ACs contain metal ions but not organic cofactors, and use ATP to activate substrates through phosphorylation. The first structural rationale for acetone carboxylation is presented here, focusing on the 360 kDa (αβγ)2 heterohexameric AC from Xanthobacter autotrophicus in the ligand-free, AMP-bound, and acetate coordinated states. Like many carboxylases, AC is a heteromultimeric enzyme complex. Its architecture consists of two heterotrimeric αβγ subunits joined by the interacting α-subunits to form a dimeric core.

In the absence of bound substrates or nucleotides (ligand-free form), the AC structure has an open cleft at the α/β subunit interface leading to the nucleotide-binding site in the β-subunit. The ligand-free structure is assigned as the resting state awaiting the binding of substrates ATP, acetone, and bicarbonate at the nucleotide-binding site. The ligand-free form of AC contains α-Glu89 positioned at the C-terminus of a Mn-proximal α-helix (residues α82–87) which blocks access to the Mn active site from the α/β interface. However, the structure of the native AC shows the nucleotide binding site located ~40 Å from the Mn site of acetoacetate formation, with no visible pathway for the transfer of reactive phosphorylated intermediates.

>[2x]MNVTVDQSTLAGATRGIVRGGETLKEHRDRLMAATKATGRYAGLKTLELREREPILYNKLFSRLRAGVVDARETAKKIAASPIVEQEGELCFTLYNAAGDSLLTSTGIIIHVGTMGAAIKYMIENNWEANPGVHDKDIFCNNDSLIGNVHPCDIHTIVPIFWEGELIGWVGGVTHVIDTGAVGPGSMATGQVQRFGDGYSITCRKVGANDTLFRDWLHESQRMVRTTRYWMLDERTRIAGCHMIRKLVEEVVAEEGIEAYWKFAYEAVEHGRLGLQARIKAMTIPGTYRQVGFVDVPYAHEDVRVPSDFAKLDTIMHAPCEMTIRRDGTWRLDFEGSSRWGWHTYNAHQVSFTSGIWVMMTQTLIPSEMINDGAAYGTEFRLPKGTWMNPDDRRVAFSYSWHFLVSAWTALWRGLSRSYFGRGYLEEVNAGNANTSNWLQGGGFNQYDEIHAVNSFECAANGTGATAVQDGLSHAAAIWNPEGDMGDMEIWELAEPLVYLGRQIKASSGGSGKYRGGCGFESLRMVWNAKDWTMFFMGNGHISSDWGLMGGYPAASGYRFAAHKTNLKELIASGAEIPLGGDTDPENPTWDAMLPDAQIKRDKQAITTEEMFSDYDLYLNYMRGGPGFGDPLDREPQAVADDINGGYVLERFAGEVYGVVVRKGADGQYGVDEAGTAAARAQIRKDRLAKSVPVSEWMKGEREKILAKDAGTQVRQMFAASFKLGPRFEKDFRTFWSLPDSWTLPEEEIGVPTYGSRYSMDISELPDVHTVQFVEE;>[2x]MHHHHHHSSGMNVPVGHLRNVQVLGIDAGGTMTDTFFVDQDGDFVVGKAQSTPQNEALGLIASSEDGLANWGMSLHEALAQLQTGVYSGTAMLNRVVQRKGLKCGLIVNRGMEDFHRMGRAVQSHLGYAYEDRIHLNTHRYDPPLVPRHLTRGVVERTDMIGTQVIPLREDTARDAARDLIAADAEGIVISLLHSYKNPENERRVRDIVLEEVEKSGKKIPVFASADYYPVRKETHRTNTTILEGYAAEPSRQTLSKISNAFKERGTKFDFRVMATHGGTISWKAKELARTIVSGPIGGVIGAKYLGEVLGYKNIACSDIGGTSFDVALITQGEMTIKNDPDMARLVLSLPLVAMDSVGAGAGSFIRLDPYTRAIKLGPDSAGYRVGVCWKESGIETVTISDCHMVLGYLNPDNFLGGAVKLDRQRSVDAIKAQIADPLGLSVEDAAAGVIELLDSDLRDYLRSMISGKGYSPASFVCFSYGGAGPVHTYGYTEGLGFEDVIVPAWAAGFSAFGCAAADFEYRYDKSLDINMPTETPDTDKEKAAATLQAAWEELTKNVLEEFKLNGYSADQVTLQPGYRMQYRGQLNDLEIESPLAQAHTAADWDQLTDAFNATYGRVYAASARSPELGYSVTGAIMRGMVPIPKPKIPKEPEEGETPPESAKIGTRKFYRKKRWVDAQLYHMESLRPGNRVMGPAVIESDATTFVVPDGFETWLDGHRLFHLREV;>MAYTRSKIVDLVDGKIDPDTLHQMLSTPKDPERFVTYVEILQERMPWDDKIILPLGPKLFIVQQKVSKKWTVRCECGHDFCDWKDNWKLSARVHVRDTPQKMEEIYPRLMAPTPSWQVIREYFCPECGTLHDVEAPTPWYPVIHDFSPDIEGFYQEWLGLPVPERADA[2x]> GSHMSTPARRRLMRDFKRMKEDSPPGVSASPLPDNV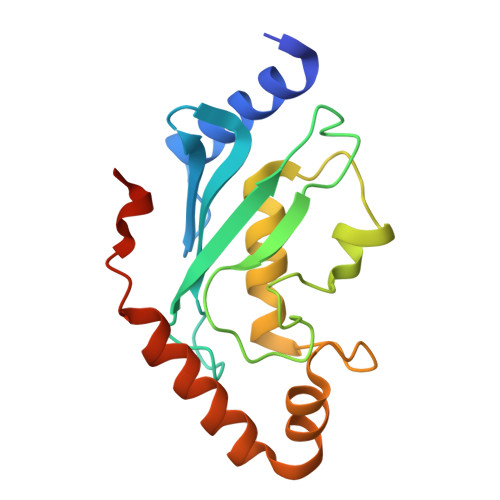MIWNAMIIGPADTPYEDGTFRLLLEFDEEYPNKPPHVKFLSEMFHPNVYANGEICLDILQNRWTPTYDVASILTSIQSLFNDPNPASPANVEAATLFQDHKSQYVKRVKETVEKSWEDDMEDMADEDEDEE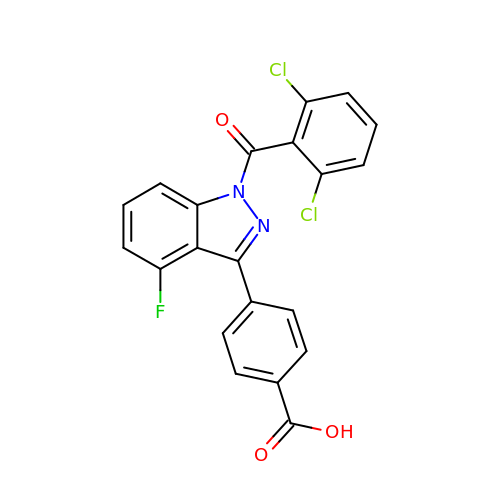4-[1-(2,6-dichlorobenzoyl)-4-fluoro-1H-indazol-3-yl]benzoic acid | C21 H11 Cl2 F N2 O3 | NEZILFWWNWEUMD-UHFFFAOYSA-N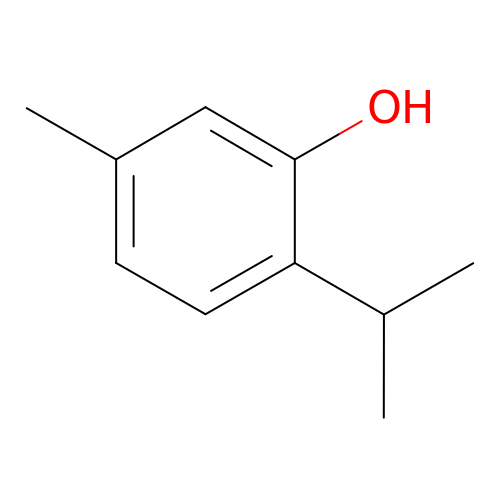5-METHYL-2-(1-METHYLETHYL)PHENOL | C10 H14 O | MGSRCZKZVOBKFT-UHFFFAOYSA-N Cytochromes P460 oxidise hydroxylamine within the nitrogen cycle and contain as their active site an unusual catalytic c-type haem where the porphyrin is crosslinked to the protein via a lysine residue in addition to the canonical cross links from cysteine residues. Cytochromes P460 consist of a homodimer with one haem P460 per monomer. The oxidation of hydroxylamine is a key part of the process of nitrification, whereby fixed nitrogen is converted to biologically available forms such as nitrate, in a range of bacteria. Here we describe the evidence for a novel double crosslink between lysine and haem in the cytochrome P460 from Methylococcus capsulatus (Bath).

Initial attempts to reduce the protein in the crystalline state using chemical reagents or by exposure to X-rays were unsuccessful as assessed by electron density (checking for movement of the iron coordinated water molecule) and crystal spectroscopy (checking for optical spectra changes that would indicate reduction). Preparation of crystals in an anaerobic glove box followed by incubation with sodium dithionite and cryotrapping resulted in successful generation of one crystal in the ferrous form as assessed by single-crystal spectroscopy of cryo-trapped crystals after reduction, Fig. 4 and S14.† The difficulty of obtaining a stable reduced form rendered it infeasible to obtain a room temperature or SFX structure of the ferrous protein. The optical absorption spectrum revealed a large spectral shift relative to the as-isolated ferric form consistent with successful reduction. Crystallographic data were measured from this reduced crystal, yielding a structure at 1.33 Å resolution. In the crystal structure, the haem distal binding position was vacant, consistent with loss of water molecule upon reduction. This results in 5-coordination of Fe(ii), which therefore moves 0.2 Å towards the proximal side of the plane of the haem. Instead, a water is 3.1 Å from the nitrogen of either pyrrole ring A or D, with an additional water 3.1 Å from the nitrogen of pyrrole ring C. Residue Lys78 only shows the single crosslink between its sidechain nitrogen and the γ-meso carbon of the haem (CHA carbon), not the crosslink between its CD carbon and the C2A carbon of the haem. The second crosslink (Lys CD–haem C2A) is broken in the crystallographic ferrous structure, causing the terminal (CMA) carbon of pyrrole ring D to change from methylene (–CH2) to methyl (–CH3). The experimental ferrous cryo structure showed a CD Lys–C2A haem distance of ∼3.7 Å, indicative of a single crosslink structure. In the ferrous cryo structure, Asp102 is the furthest from the iron centre (average 5.9 Å), consistent with proton transfer not being needed at this stage of the catalytic cycle, because no ligand is bound to the iron. However, after collection of the X-ray diffraction data (0.20 MGy dose), the peak shifted to 451 nm.

>[2x]EPAAAPNGISLPAGYKDWKMIGVSSRIEQNNLRAILGNDIAVKAAREGRTHPWPDGAILVKLSWKKSTHELFPSAEVPGDFTQADFMVKDAAKYASTGGWGYARWLGMEQKPYGANADFAQECMGCHSGAKAADYVFTHPAKLP> MHPGWPDTVGPLRVPAGVVGLRPVRMRDAAAWSRIRLADQHHLEPWEPMTGMDWKVRHAVTSWPSICSGLRAEARHGRMLPFVIELDGEFVGQLTIGNVTHGALRSAWIGYWVASSRTGGGIATAALAMGLDHCFTAVQLHRIEATVRPENTPSRAVLAHVGFREEGLL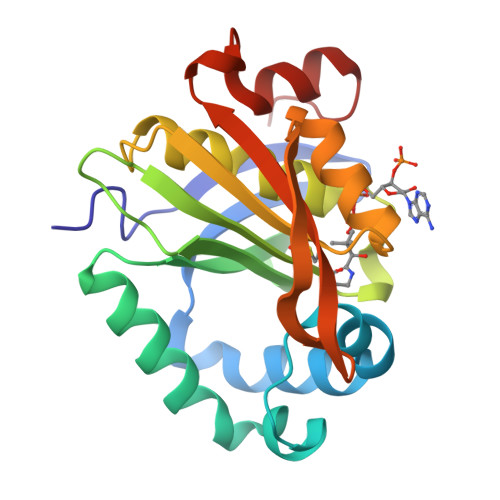KRYLEVDGAWRDHLLVAITAEELPQSAAHRLVAAGRAEWC>[2x]AYTTFSQTKNDQLKEPMFFGQPVNVARYDQQKYDIFEKLIEKQLSFFFRPEEVDVSRDRIDYQALPEHEKHIFISNLKYQTLLESIQGRSPNVALLPLISIPELETWVETWAFSETIHSRSYTHIIRNIVNDPSVVFDDIVTNEQIQKRAEGISSYYDELIEMTSYWHLLGEGTHTVNGKTVTVSLRELKKKLYLCLMSVNALEAIRFYVSFACSFAFAERELMEGN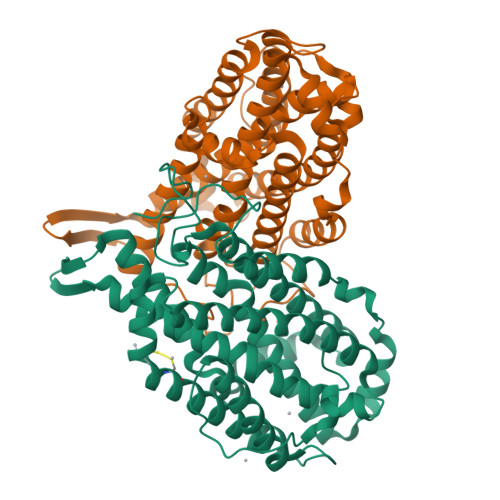AKIIRLIARDEALHLTGTQHMLNLLRSGADDPEMAEIAEECKQECYDLFVQAAQQEKDWADYLFRDGSMIGLNKDILCQYVEYITNIRMQAVGLDLPFNTRSNPIPWINTWLVSDNVQVAPQEVEVSSYLVGQIDSEVDTDDLSNFQL> DEALSRHFNELRTMGETLKYSEDLDFILSDNSMTTPEHRRNNMLRLCLDMMNNEDLCQYIVKYRHREVWEWCFQGTDPKQKVTSLLQCFIADKIPLLRHDKRWAMLSLENFILPLATDEVFPKKIAGSRLVKLNYQDLLRKLKFTNTCEYALYIWATYLLYTEAVYGAVPALARLISRGQLKDWDTACSLLENNIVAAPSGSDIEEYAQAFQTLAGLSREKLTNEGVLKCLIKLTNHTTVLELSADLLPSLVRSLAMSVQLHQNNIVSSISEIKTNLLILQLGLLLNIVSEATTAASTEELTNFGA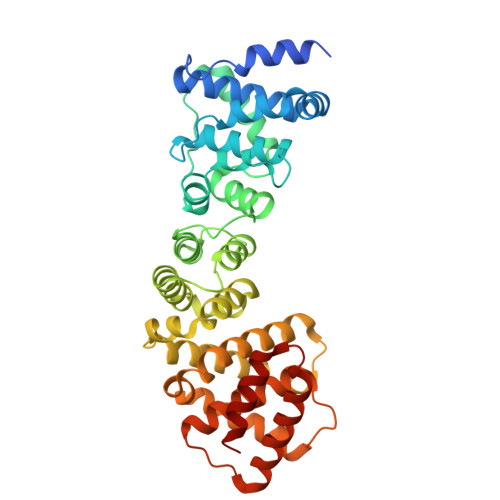VFRSVFVKKPTEMSFVLQLFLLVYAYSAGAAGVQLPPAEADFLKSELEAFATDVSSYNHNIHTRITRVLETL> GSHMASPN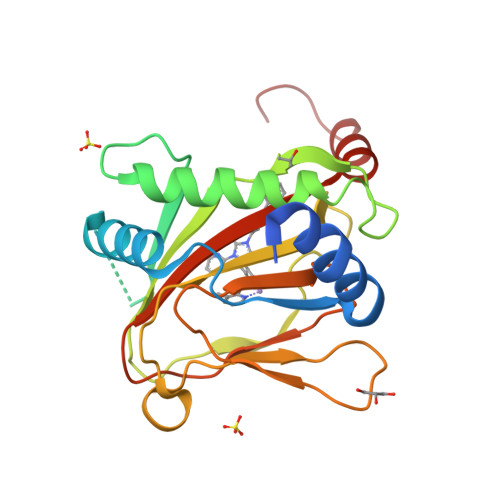GQTKPLPALKLALEYIVPCMNKHGICVVDDFLGKETGQQIGDEVRALHDTGKFTDGQLVSQKSDSSKDIRGDKITWIEGKEPGCETIGLLMSSMDDLIRHCNGKLGSYKINGRTKAMVACYPGNGTGYVRHVDNPNGDGRCVTCIYYLNKDWDAKVSGGILRIFPEGKAQFADIEPKFDRLLFFWSDRRNPHEVQPAYATRYAITVWYFDADERARAKVKYLTGE> MRGSHHHHHHGRSLNPLSTPQFDSTDETPASYNLAVRRAAPAVVNVYNRGLNTNSHNQLEIRTLGSGVIMDQRGYIITNKHVINDADQIIVALQ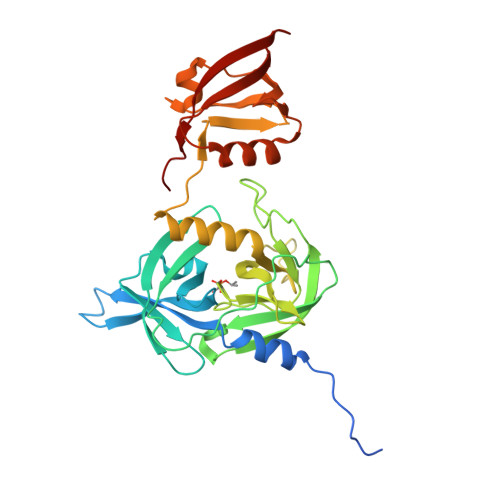DGRVFEALLVGSDSLTDLAVLKINATGGLPTIPINARRVPHIGDVVLAIGNPYNLGQTITQGIISATGRIGLNPTGRQNFLQTDASINPGNSGGALVNSLGELMGINTLSFDKSNDGETPEGIGFAIPFQLATKIMDKLIRDGRVIRGYIGIGGREIAPLHAQGGGIDQLQGIVVNEVSPDGPAANAGIQVNDLIISVDNKPAISALETMAQVAEIRPGSVIPVVVMRDDKQLTLQVTIQEYPATN>[3x]MNNQIFESVDHYISDLLGYEDDALLAATNSLAEAGMPAISVSPNQGKFLQLLAQLCQAKNILELGTLAGYSTIW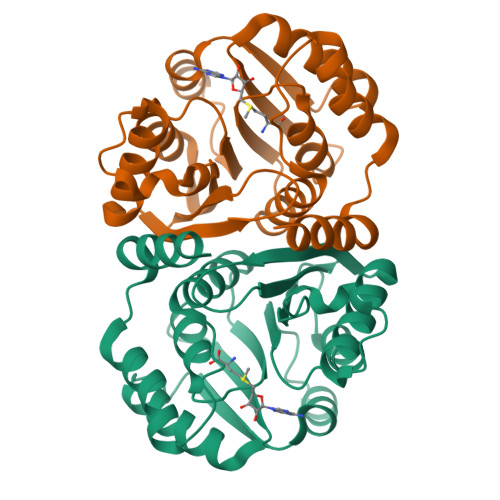MARALPKNGRLITLEYDPKHAAVAQKNIDRAGLTSQVQIRTGKAIDILPQLVEEGAGPFDMIFIDADKPPYTEYFQWALRLSRPGTLIVADNVIRDGKVLDENSTEPAVQGARRFNAMLGANTAVDATILQMVGVKEYDGMALAIVKLEHHHHHH>[4x]SDKIIHLTDDSFDTDVLKADGAILVDFWAE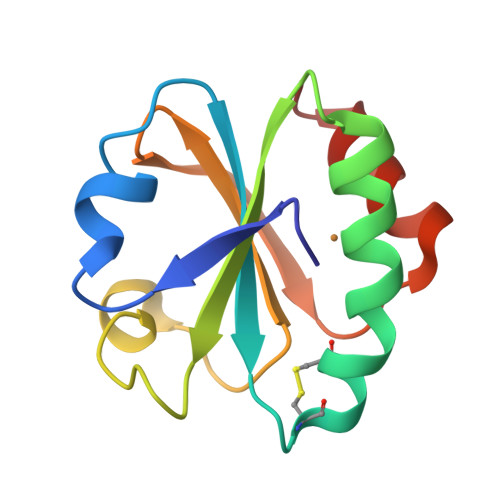WCGPCKMIAPILDEIADEYQGKLTVAKLNIDQNPGTAPKYGIRGIPTLLLFKNGEVAATKVGALSKGQLKCFLDCNLA3,4-difluorobenzamide | C7 H5 F2 N O | 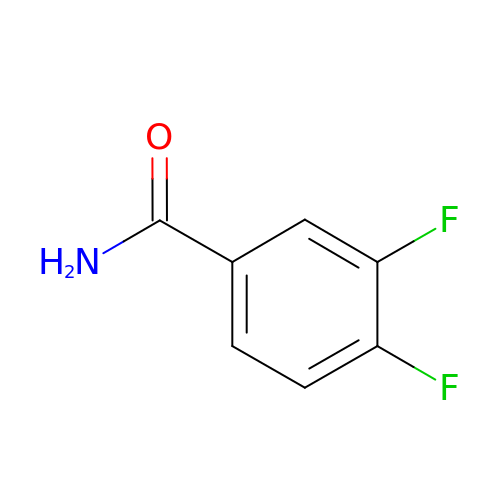CMWOHNIHUBDEAG-UHFFFAOYSA-N>[2x]MKNATFYLLDNDTTVDGLSAVEQLVCEIAAERWRSGKRVLIACEDEKQAYRLDEALWARPAESFVPHNLAGEGPRGGAPVEIAWPQKRSSSRRDILISLRTSFADFATAFTEVVDFVPYEDSLKQLARERYKAYRVAGFNLNTATWK;>[2x]QGEIAIAIPAHVRLVMVANDLPALTDPLVSDVLRALT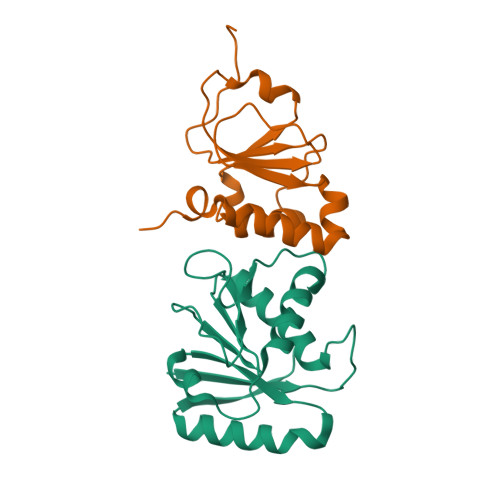VSPDQVLQLTPEKIAMLPQGSHCNSWRLGTDEPLSLEGAQVASPALTDLRANPTARAALWQQICTYEHDFFPRND> GKAFDDGAFTGIREINLSYNKETAIGDFQVVYDLNGSPYVGQNHSSFISGFTPVKISLDFPSEYITEVSGYTGNVSGYVVVRSLTFKTNKKTYGPYGVTSGTPFNLPIENGLIVG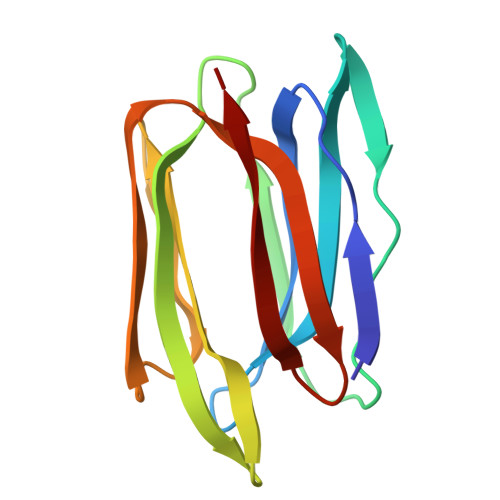FKGSIGYWMDYFSMYLSL>MATKGTKRSYEQMETDGERQNATEIRASVGKMIDGIGRFYIQMCTELKLSDYEGRLIQNSLTIERMVLSAFDERRNKYLEEHPSAGKDPKKTGGPIYRRVDGKWRRELILYDKEEIRRIWRQANNGDDATAGLTHMMIWHSNLNDATYQRTRALVRTGMDPRMCSLMQGSTLPRRSGAAGAAVKGVGTMVMELIRMIKRGINDRNFWRGENGRRTRIAYERMCNILKGKFQTAAQRTMVDQVRESRNPGNAEFEDLIFLARSALILRGSVAHKSCLPACVYGSAVASGYDFEREGYSLVGIDPFRLLQNSQVYSL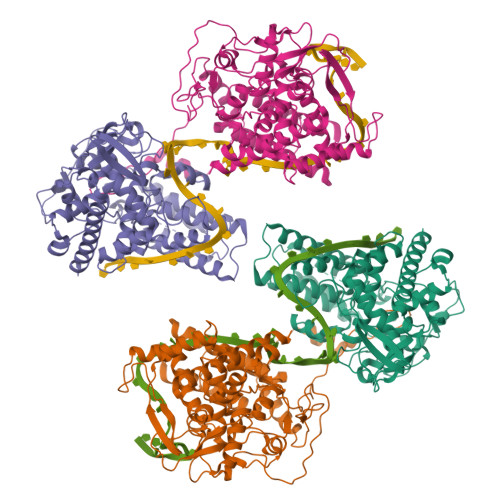IRPNENPAHKSQLVWMACHSAAFEDLRVSSFIRGTKVVPRGKLSTRGVQIASNENMETMESSTLELRSRYWAIRTRSGGNTNQQRASSGQISIQPTFSVQRNLPFDRPTIMAAFTGNTEGRTSDMRTEIIRLMESARPEDVSFQGRGVFELSDEKATSPIVPSFDMSNEGSYFFGDNAEEYDN[4x]>MSGIALSRLAQERKAWRKDHPFGFVAVPTKNPDGTMNLMNWECAIPGKKGTPWEGGLFKLRMLFKDDYPSSPPKCKFEPPLFHPNVYPSGTVCLSILEEDKDWRPAITIKQILLGIQELLNEPNIQDPAQAEAYTIYCQNRVEYEKRVRAQAKKFAPS[2x];> AEPVQEELSVLAAIFCRPHEWEVLSRSETDGTVFRIHTKAEGFMDVDIPLELVFHLPVNYPSCLPGISINSEQLTRAQCVTVKEKLLEQAESLLSEPMV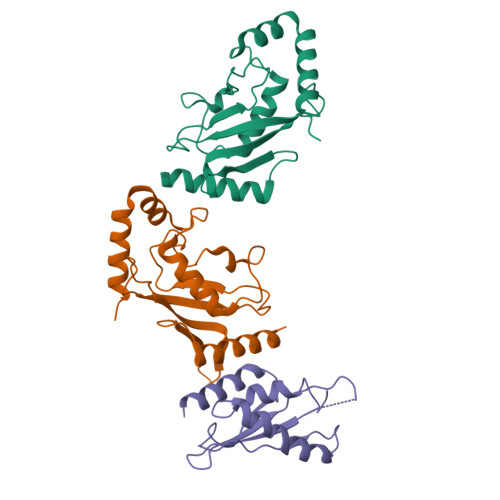HELVLWIQENLRHA>[7x]MRNDTRRLFAAYKAAIAKLNGVERVDEKFSVAPSVQQKLETKVQESSDFLKSINFYGVPEQEGEKIGLGVSGPVASTTDTTQQDRETSDISTMDGRRYRCEQTNSDTHITYQKLDAWAKFADFQTRIRDAIIKRQALDRIMIGFNGVSRAATSDRVANPMLQDVNK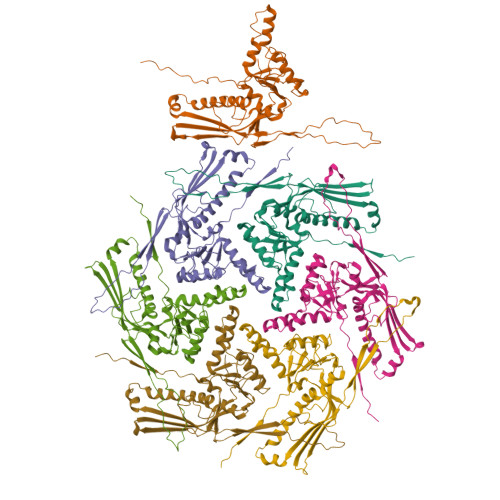GWLQNLREQAPQRVMKEGKAAAGKITVGGAGADYGNLDALVYDITNHLVEPWYAEDPDLVVVCGRNLLSDKYFPLVNRDRDPVQQIAADLIISQKRIGNLPAIRVPYFPANGLLVTRLDNLSIYYQEGGRRRTILDNAKRDRIENYESSNDAYVIEDLACAAMAENIALAAAA>ATAAQAERTLPKKYGGRFTVTLIPGDGVGKEITDSVRTIFEAENIPIDWETINIKQTDHKEGVYEAVESLKRNKIGLKGLWHTPADQTGHGSLNVALRKQLDIYANVALFKSLKGVKTRIPDIDLIVIRENTEGEFSGLEHESVPGVVESLKVMTRPKTERIARFAFDFAKKYNRKSVTAVHKANIMKLGDGLFRNIITEIGQKEYPDIDVSSIIVDNASMQAVAKPHQFDVLVTPSMYGTILGNIGAALIGGPGLVAGANFGRDYAVFEPGSRHVGLDIKGQNVANPTAMILSSTLMLNHLGLNEYATRISKAVHETIAEGKHTTRDIGGSSSTTDFTNEIINKLSTM[8x];>[8x]ATVKQPSIGRYTGKPNPSTGKYTVSFIEGDGIGPEISKSVKKIFSAANVPIEWESCDVSPIFVNGLTTIPDPAVQSITKNLVALKGPLATPIGKGHRSLNLTLRKTFGLFANVRPAKSIEGFKTTYENVDLVLIRENTEGEYSGIEHIVCPGVVQSIKLITRDASERVIRYAFEYARAIGRPRVIVVHKSTIQRLADGLFVNVAKELSKEYPDLTLETELIDNSVLKVVTNPSAYTDAVSVCPNLYGDILSDLNSGLSAGSLGLTPSANIGHKISIF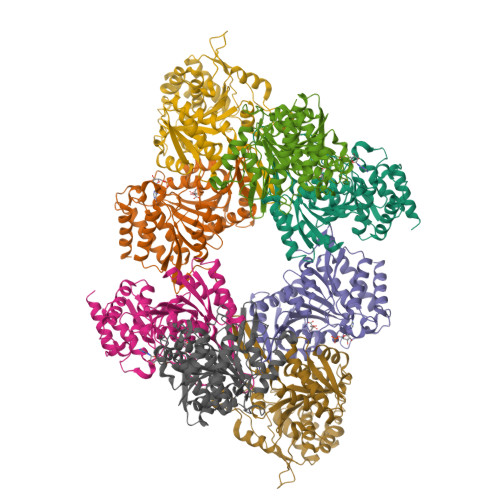EAVHGSAPDIAGQDKANPTALLLSSVMMLNHMGLTNHADQIQNAVLSTIASGPENRTGDLAGTATTSSFTEAVIKRL>[2x]MRQLAKDINAFLNEVILQAENQHEILIGHCTSEVALTNTQEHILMLLSEESLTNSELARRLNVSQA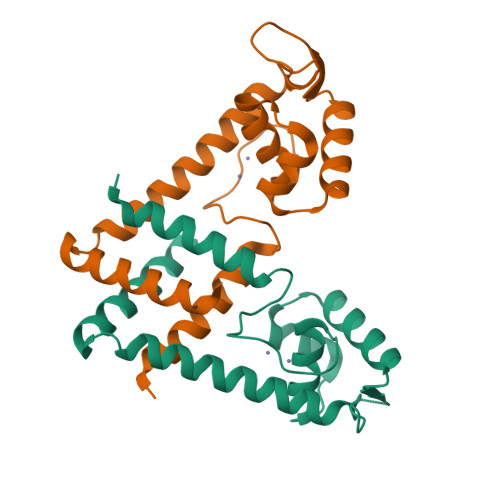AVTKAIKSLVKEGMLETSKDSKDARVIFYQLTDLARPIAEEHHHHHEHTLLTYEQVATQFTPNEQKVIQRFLTALVGEIK>GPGMAVKHLIVLKFKDEITEAQKEEFFKTFVNLVNIIPAMKDVYWGKDVTQKNKEEGYTHIVEVTFESVETIQDYIIHPAHVG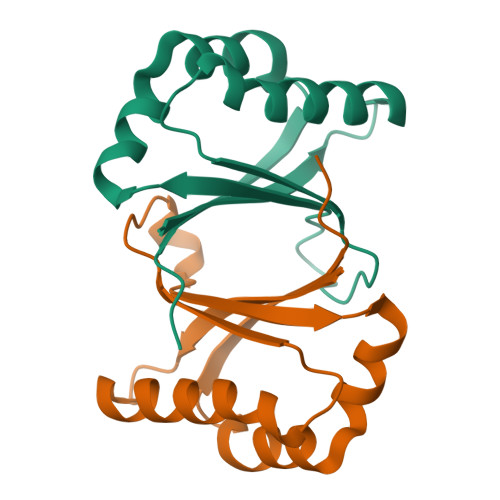FGDVYRSFWEKLLIFDYTPRK[2x]> AEFMEEYQKFTNESLLWAPYRSNCYFGMRPRYVHESPLIMGIMWFNSLSQDGLHSLRHFATPQDKLQKYGWEVYDPRIGGKEVFIDEKNNLNLTVYFVKSKNGENWSVRVQGEPLDPKRPSTASVVLYFSQNGGEIDGKSSLAMIGHDGPNDMKFFGYSKELGEYHLTVKDNFGHYFKNPEYETMEVAPGSDCSKTSHLSLQIPDKEVWKARDVFQSLVSDSIRDILEKEETKQRPADLIPSVLTIRNLYNFNPGNFHYIQKTFDLTKKDGFQFDITYNKLGTTQSISTREQVTELITWSLNEINARFDKQFSFGEGPDSIESVEVKRRFALETLSNLLGGIGYFYGNQLIDRETEFDESQFTEIKLLNAKEEGPFELFTSVPSRGFFPRGFYWDEGFHLLQIMEYDFDLAFEILASWFEMIEDDSGWIAREIILGNEARSKVPQEFQVQNPNIANPPTLLLAFSEMLSRAIENIGDFNSDSYHQVMFNSRTAKFMTNNLEANPGLLTEYAKKIYPKLLKHYNWFRKSQTGLIDEYEEILEDEGIWDKIHKNEVYRWVGRTFTHCLPSGMDDYPRAQPPDVAELNVDALAWVGVMTRSMKQIAHVL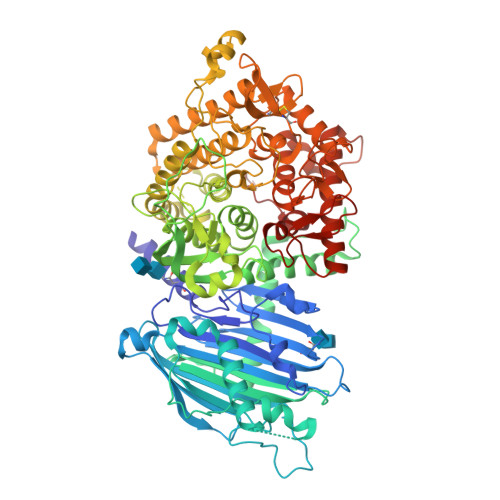KLTQDEQRYAQIEQEVVENLDLLHWSENDNCYCDISIDPEDDEIREFVCHEGYVSVLPFALKLIPKNSPKLEKVVALMSDPEKIFSDYGLLSLSRQDDYFGKDENYWRGPIWMNINYLCLDAMRYYYPEVILDVAGEASNAKKLYQSLKINLSNNIYKVWEEQGYCYENYSPIDGHGTGAEHFTGWTALVVNILGRFRSHHHHHH>[2x]MASWSHPQFEKGAVTSLYKKAGFQK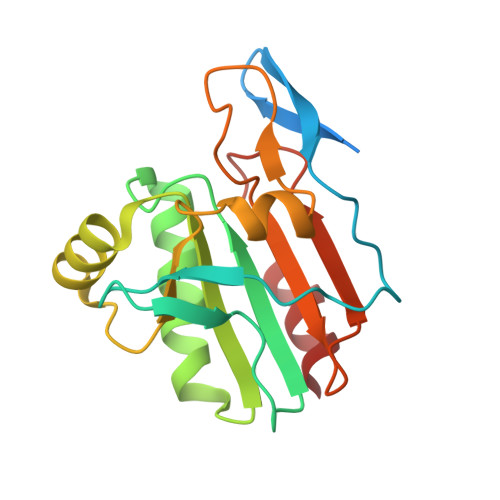VTFKEETYQLEGKALKVGDKAPDVKLVNGDLQEVNLLKQGVRFQVVSALPSLTGSVCLLQAKHFNEQTGKLPSVSFSVISMDLPFSQGQICGAEGIKDLRILSDFRYKAFGENYGVLLGKGSLQGLLARSVFVLDDKGVVIYKEIVQNILEEPNYEALLKVLK>[6x]SNAMTIKGRAFPEGFLWGGAVAAHQLEGGYKEGGKGLSTADIMTLGTNERPREITDGVVAGKYYPNHQAIDFYHRYPEDIELFAEM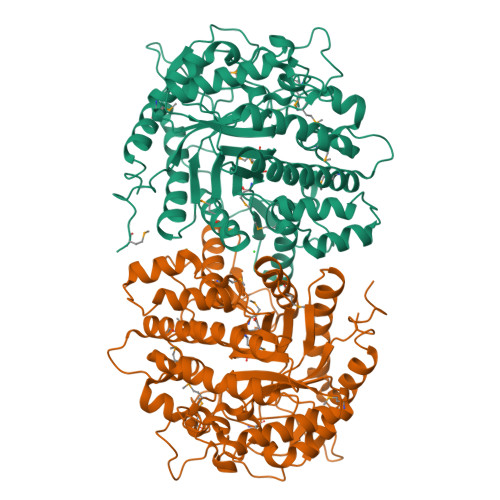GFKCFRTSIAWTRIFPNGDESEPNEAGLQFYDDLFDECLKNGIQPVVTLAHFEMPYHLVKQYGGWRNRKLIQFYLNFAKVCFERYRDKVTYWMTFNEINNQTNFESDGAMLTDSGIIHQPGENRERWMYQAAHYELVASAAAVQLGHQINPDFQIGCMIAMCPIYPLTAAPADVLFAQRAMQTRFYFADVHCNGTYPQWLRNRFESEHFNLDITAEDLKILQAGTVDYIGFSYYMSFTVKDTGKLAYNEEHDLVKNPYVKASDWGWQVDPVGLRYAMNWFTDRYHLPLFIVENGLGAIDKKTADNQIHDDYRIDYLTDHLRQIKLAVLEDGVDLIGYTPWGCIDLVAASTGQMSKRYGFIYVDENDDGSGSLKRYKKDSFTWFQHVIATNGAEIE>MAHHHHHHMISFYGYTHFDGRTLKNKYGMQGKALQERCAYDLLQAMLNLRKEPLPEKFDSSYLKYLHQRLYEKMFEWAGCTCDTPFTFSDGTVTKVPINNKIKEGLKRIDQILAEKNNFQGLSRKEFIHEVSTVFILLNKI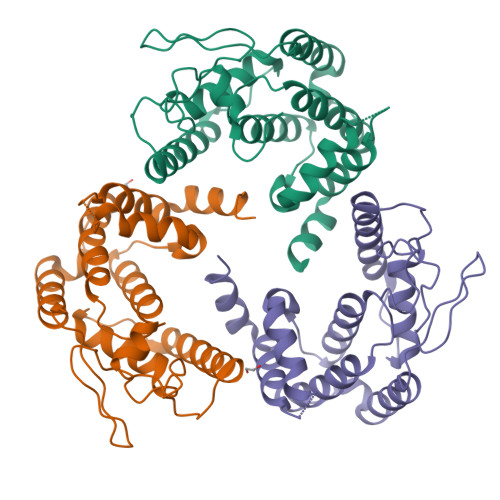RPFMVGNKYVQRIFFEQIAEAAGHKLDFSVVTEKRMQFAIHAALSFDGNNNRGNITPMLHLFEDISNPEKVGILKEFMIYI[6x]Mitogen-activated protein kinase kinase kinase kinase 1 (MAP4K1) is a serine/threonine kinase that acts as an immune checkpoint downstream of T-cell receptor stimulation. MAP4K1 activity is enhanced by prostaglandin E2 (PGE2) and transforming growth factor beta (TGFβ), immune modulators commonly present in the tumor microenvironment. Therefore, its pharmacological inhibition is an attractive immuno-oncology concept for inducing therapeutic T-cell responses in cancer patients. Through its proline-rich domain, MAP4K1 binds to a diversity of adaptors in hematopoietic cells, including those involved in T-cell receptor (TCR), B-cell receptor, and cytokine-induced signaling. The function of MAP4K1 has been studied most extensively in the context of T-cell activation.

Protein X-ray crystallography confirmed that the urea moiety interacts in a bidentate hydrogen bond with the Asp101 side chain in MAP4K1 (Asp112 in the surrogate kinase MST1). Ureas synthesized from cyclic amines, which reduced overall H-bond donors by one (not shown), also displayed more than a 10-fold decrease in activity, highlighting the importance of the two hydrogen bonds for overall potency.

>GMETVQLRNPPRRQLKKLDEDSLTKQPEEVFDVLEKLGEGSYGSVYKAIHKETGQIVAIKQVPVESDLQEIIKEISIMQQCDSPHVVKYYGSYFKNTDLWIVMEYCGAGSVSDIIRLRNKTLTEDEIATILQSTLKGLEYLHFMRKIHRDIKAGNILLNTEGHAKLADFGVAGQLTDTMAKRNTVIGTPFWMAPEVIQEIGYNCVADIWSLGITAIEMAEGKPPYADIHPMRAIFMIPTNPPPTFRKPELWSDNFTDFVKQCLVKSPEQRATATQLLQHPFVRSAKGVSILRDLINEAMDVKLKRQESQQRE[2x]>MSANDRRDRRVRVAVVFGGRSNEHAISCVSAGSILRNLDSRRFDVIAVGITPAGSWVLTDANPDALTITNRELPQVKSGSGTELALPADPRRGGQLVSLPPGAGEVLESVDVVFPVLHGPYGEDGTIQGLLELAGVPYVGAGVLASAVGMDKEFTKKLLAADGLPVGAYAVLRPPRSTLHRQECERLGLPVFVKPARGGSSIGVSRVSSWDQLPAAVARARRHDPKVIVEAAISGRELECGVLEMPDGTLEASTLGEIRVAGVRGREDSFYDFATKYLDDAAELDVPAKVDDQVAEAIRQLAIRAFAAIDCRGLARVDFFLTDDGPVINEINTMPGFTTISMYPRMWAASGVDYPT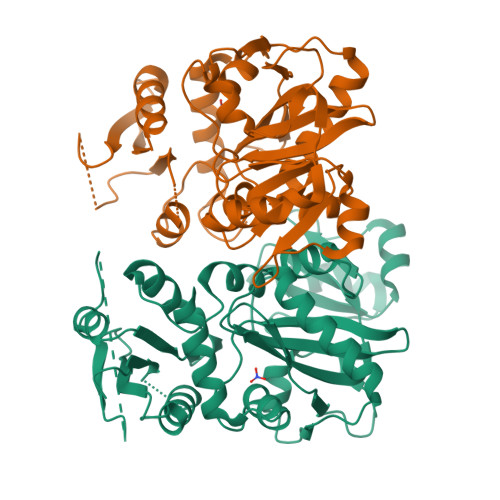LLATMIETTLARGVGLH[2x]> VREILSIHVGQCGNQIADSFWRLALREHGLTEAGTLKEGSNAAANSNMEVFFHKVRDGKYVPRAVLVDLEPGVIARIEGGDMSQLFDESSIVRKIPGAANNWARGYNVEGEKVIDQIMNVIDSAVEKTKGLQGFLMTHSIGGGSGSGLGSLILERLRQAYPKKRIFTFSVVPSPLISDSAVEPYNAILTLQRILDNADGAVLLDNEALFRIAKAKLNRSPNYMDLNNIIALIVSSVTASLRFPGKLNTDLSEFVTNLVPFPGNHFLTASFAPMRGAGQEGQVRTNFPDLARETFAQDNFTAAIDWQQGVYLAASALFRGDVKAKDVDENMA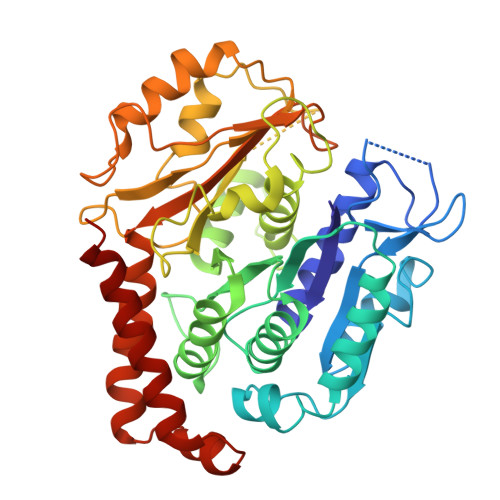TIRKSLNYASYMPASGGLKLGYAETAPEGFASSGLALVNHTGIAAVFERLIAQFDIMFDNHAYTHWYENAGVSRDMMAKARNQIATLAQSYRDAS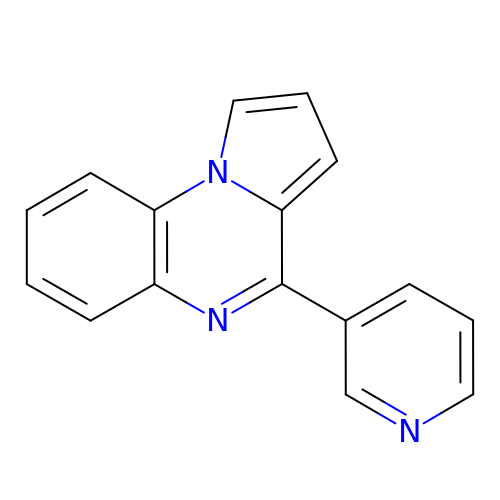4-pyridin-3-ylpyrrolo[1,2-a]quinoxaline | C16 H11 N3 | YYLFSLFSCWVKLI-UHFFFAOYSA-N> AVGTGIPEGSLQFLSLRASAPIGSAISRNNWAVTCDSAQSGNECNKAIDGNKDTFWHTFYGANGDPKPPHTYTIDMKTTQNVNGLSMLPRQDGNQNGWIGRHEVYLSSDGTNWGSPVASGSWFADSTTKYSNFETRPARYVRLVAITEANGQPWTSIAEINVFQASSYTAPQPGLGRWGPTIDLPIVPAAAAIEPTSGRVLMWSSYRNDAFGGSPGGITLTSSWDPSTGIVSDRTVTVTKHDMFCPGISMDGNGQIVVTGGNDAKKTSLYDS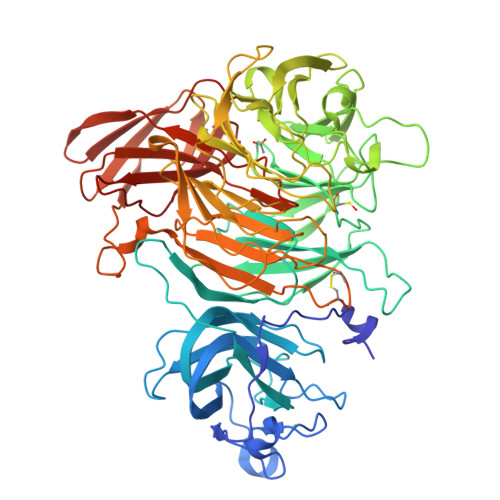SSDSWIPGPDMQVARGYQSSATMSDGRVFTIGGSWSGGVFEKNGEVYSPSSKTWTSLPNAKVNPMLTADKQGLYRSDNHAWLFGWKKGSVFQAGPSTAMNWYYTSGSGDVKSAGKRQSNRGVAPDAMCGNAVMYDAVKGKILTFGGSPDYQDSDATTNAHIITLGEPGTSPNTVFASNGLYFARTFHTSVVLPDGSTFITGGQRRGIPFEDSTPVFTPEIYVPEQDTFYKQNPNSIVRVYHSISLLLPDGRVFNGGGGLCGDCTTNHFDAQIFTPNYLYNSNGNLATRPKITRTSTQSVKVGGRITISTDSSISKASLIRYGTATHTVNTDQRRIPLTLTNNGGNSYSFQVPSDSGVALPGYWMLFVMNSAGVPSVASTIRVTQ>SNALSEVSEGNDIDRHLVRQMTVLSQGNDQYFRFVTRLSRAMDVKIGGGTPDFAPARQSLENMRQKLEEMKALSPGPMNPDISREVLSNWQALL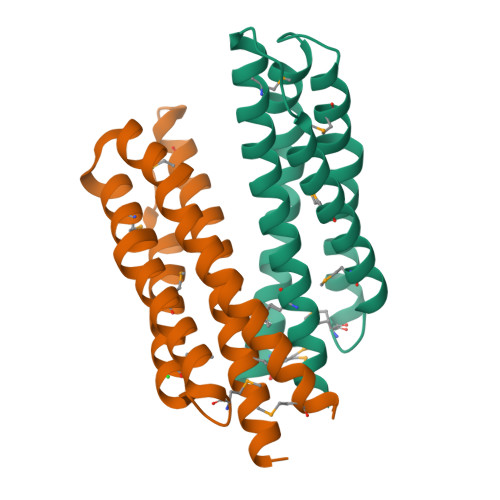EKGVVPQMQLAQQGSLTAWSEHASTVTPALSRAFGASAERFSHEAGAMLDNTRVMVDGKTYTIR[2x]Herein, we describe the biochemical and structural characterization of two multi-FMN-containing covalent flavoproteins, SaFMN3 from Streptomyces azureus and CbFMN4 from Clostridiaceae bacterium. Based on their primary structure, these proteins were predicted to contain three and four covalently tethered FMN cofactors, respectively. Recently, Méheust et al. discovered by sequence analysis a multitude of sequences of extracytosolic proteins predicted to contain multiple covalently bound FMN molecules. Such multi-FMN binding proteins are thought to play a role in extracellular long-distance electron transfer paths similar to multi-heme proteins. The crystal structures were elucidated, which confirmed that the flavin cofactor is covalently attached to a threonine.

The second domain of SaFMN3 (SaFMN3-D2, residues 157–244) and the first domain of CbFMN4 (CbFMN4-D1, residues 26–109) could be overexpressed as soluble proteins. The SaFMN3-D2 (9.4 kDa) structural organization consists of three β-strands forming an anti-parallel sheet (residues 2–6, 18–24 and 27–35), followed by two α-helices (residues 41–60 and 72–87) connected by a loop. The FMN-binding site is located between the N-terminal parts of the first helix and second helix. Most prominent is the hydrophobic stacking interaction of Tyr14 on the si-face of the isoalloxazine and Ile45 on its re-face. Furthermore, hydrogen bonds are located between the O2 of FMN and the backbone amides of Tyr73 and Thr74, the N3 with the Thr74-Oγ1, and the N5 with the Oγ of Ser42. The phosphate group of the FMN is clearly covalently attached to the Oγ1 of Thr72, which is located at the start of the last α-helix. The structure of SaFMN3-D2 shows that FMN closely interacts with the side chains of Tyr14, Ile45, and Tyr73. Especially the benzylic moiety of the isoalloxazine is sandwiched between Ile45 and Tyr14, which may lead to quenching of fluorescence. The highest fluorescence quantum yield among all mutants was 0.07 for SaFMN3-D2-Tyr14Ala/Tyr73Ala and SaFMN3-D2-Tyr14Ala/Tyr73Ala/Ile45Ala. These data suggest that the Tyr14 and Tyr73 side chains have a fluorescence quenching effect on the bound FMN. When inspecting the crystal structure of the SaFMN3-D2, no clear binding pocket next to the isoalloxazine moiety can be identified that could bind an organic substrate.

> MAQTVTGDVAQTQYGPVQVRITVAGGKITKAEAVQAPKGGRSDQITSASVPRLNQAAVAAGSAEIDAVSGATYTSAGYKKSLQSALDKA> MELLFLGTGAGIPAKARNVTSVALKLLEERRSVWLFDCGEATQHQMLHTTIKPRKIEKIFITHMAGDHVYGLPGLLGSRSFQGGEDELTVYGPKGIKAFIETSLAVTKTHLTYPLA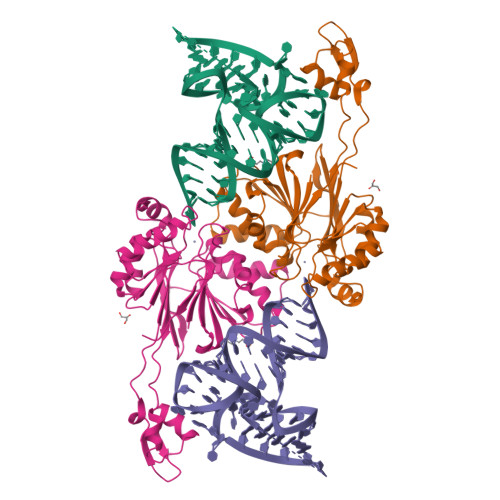IQEIEEGIVFEDDQFIVTAVSVIHGVEAFGYRVQEKDVPGSLKADVLKEMNIPPGPVYQKIKKGETVTLEDGRIINGNDFLEPPKKGRSVVFSGDTRVSDKLKELARDCDVMVHEATFAKEDRKLAYDYYHSTTEQAAVTAKEARAKQLILTHISARYQGDASLELQKEAVDVFPNSVAAYDFLEVNVPRGKLAAALEHHHHHH>MENFIGSHMIYTYENGWEAEIYIKNDHTIDYRIHSGMVAGRWVRDQEVNIVKLTEGVYKVSWTEPTGTDVSLNFMPNEKR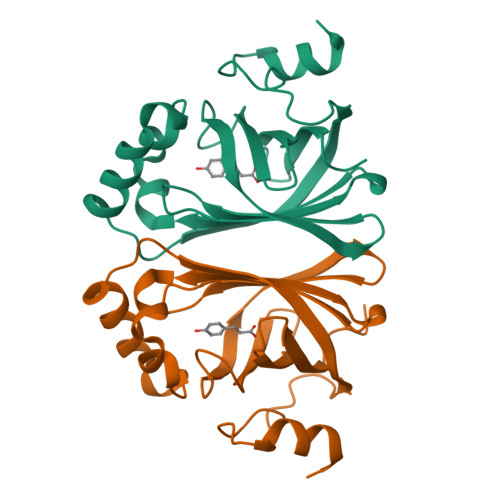MHGIIFFPKWVHEHPEITVCYQNDHIDLMKESREKYETYPKYVVPEFAEITFLKNEGVDNEEVISKAPYEGMTDDIRAGRL[3x]>[4x]SMRKTIERLLNSELSSNSIAVRTGVSQAVISKLRNGKKELGNLTLNSAEKLFEYQKEMEKVDTWIVYRGR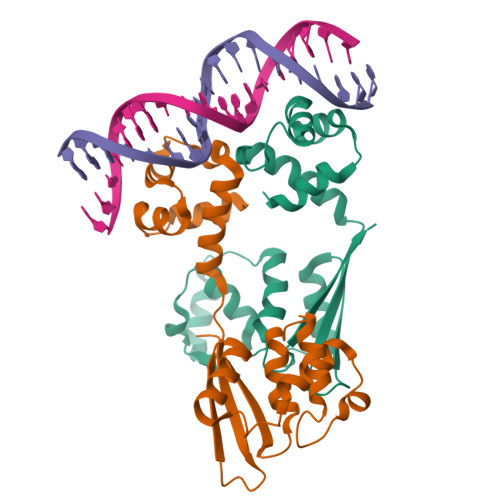TADMNKSYIAEGSTYEEVYNNFVDKYGYDVLDEDIYEIQLLKKNGENLDDYDVDSDGINNYDKLDEFRESDYVDLEDYDYRELFENSSSQVYYHEFEITHE> MASAHIALELDKTKVKVGDVIVATVKAKNMTSMAGIQVNIKYDPEVLQAIDPATGKPFTKETLLVDPELLSNREYNPLLTAVNDINSGIINYASCYVYWDSYRESGVSESTGIIGKVGFKVLKAANTTVKLEETRFTPNSIDGTLVIDWYGQQIVGYKVIQPDLEHHHHHH;> MNKPVIE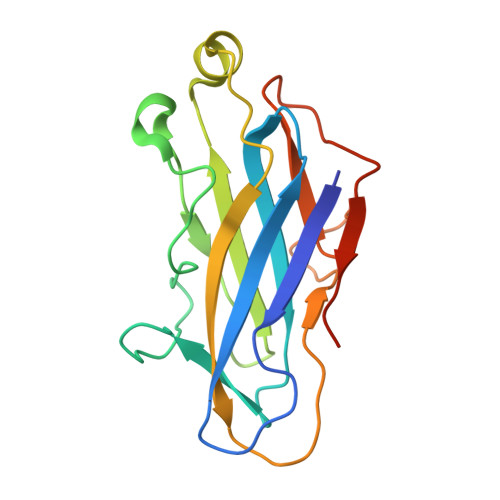GYKVSGYILPDFSFDATVAPLVKAGFKVEIVGTELYAVTDANGYFEITGVPANASGYTLKISRATYLDRVIANVVVTGDTSVSTSQAPIMMWVGKIVKDNSINLLDVAEVIRCFNATKGSANYVEELDINRNGAINMQDIMIVHKHFGATSSDYDAQ> ASWSHPQFEKSGGGGGLVPRGSGSSCWQSNSAYEINMAMGRVVVSPDLPVGSVIATKTWTMPDNNTIYVTCDRNTTLKSDAKVVAAGLVQGANKVYSTAIPGIGLRFSRKGAISMIYPDSYTTTGSSFRLAGSTFTLDIIKTSTTTGSGTLASGPYTEYGPGFTILKTSLNADAITIVSPS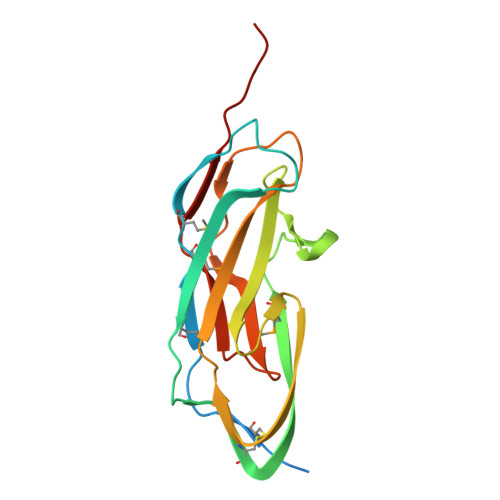CTIL> MQ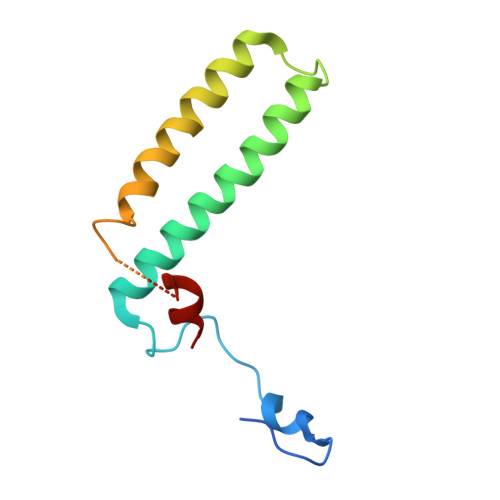KHNIKLNQNQDISQLFHDEVPLFDNSITSKDKEVIETLSEIYSIVITLDHVEKAYLKDSIDDTQYTNTVDKLLKQFKVYLNSQNKEEINKHFQSIEAFADTYNITASNAITRLERG>[15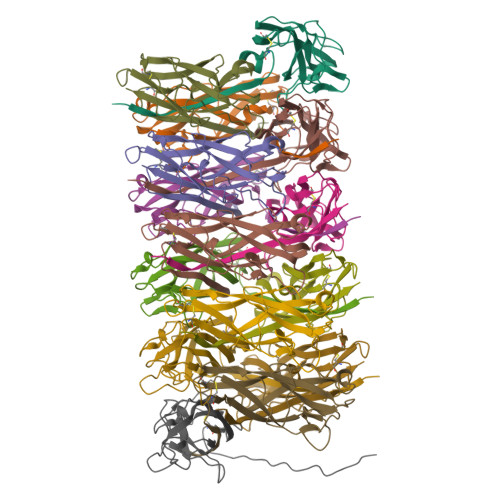x]AATTVNGGTVHFKGEVVNAACAVDAGSVDQTVQLGQVRTASLAQEGATSSAVGFNIQLNDCDTNVASKAAVAFLGTAIDAGHTNVLALQSSAAGSATNVGVQILDRTGAALTLDGATFSSETTLNNGTNTIPFQARYFATGAATPGAANADATFKVQYQ N-(5-ethyl-1,2-oxazol-3-yl)-N'-[4-(2-{[6-(4-ethylpyrazin-1(4H)-yl)pyrimidin-4-yl]amino}-1,3-thiazol-5-yl)phenyl]urea 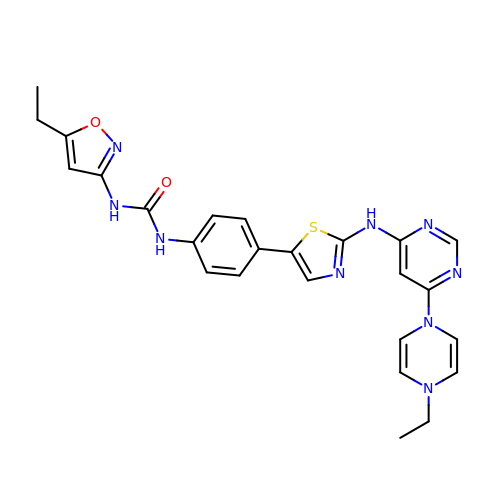| C25 H25 N9 O2 S | UPVPVNFMFOJQIG-UHFFFAOYSA-N> 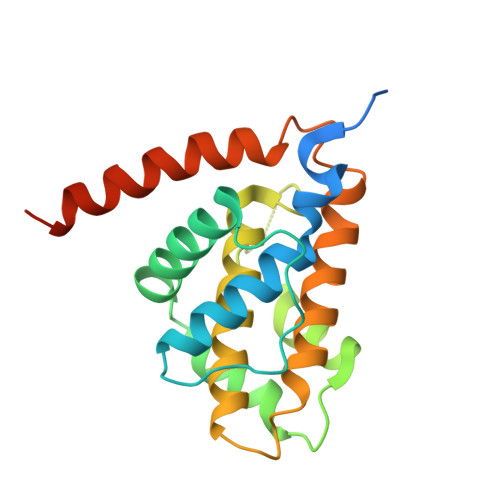LPSPSRQASTRRMSIGESIDGKINDWEEPRLDIEGFVVDYFTHRIRQNGMEWFGAPGLPSGVQPEHEMMRVMGTIFEKKHAENFETFSEQLLAVPRISFSLYQDVVRTVGNAQTDQSPMSYGRLIGLISFGGFVAAKMMESVELQGQVRNLFVYTSLFIKTRIRNNWKEHNRSWDDFMTLGKQMKEDYERAEAEKVGRRKQNRR>MTQTAAKSLKFPKDFLWGAATAAYQIEGAANEDGRGPSIWDTFSHTPGKVHNGDNGDVACDHYHRYKEDVELMKELGLNAYRFSISWPRILPEGEGKVNQKGLDFYNNLIDELLENGIEPFVTLYHWDLPQALQDKGGWENRETVDAFAEYARVCFERFGDRVKYWITFNEPNVFAVLGYLSGVHPPGMKDLKKAFRAAHNLLLAHARAVKAYREISQNGQIGITLNLSPVYPASDNEEEDKAAAERADQFNNWFLDPIFKGKYEHMLERLGEQIAANGGELPEITDEMEILSASLDFIGLNYYTSNLVRANPNSGSSSVKP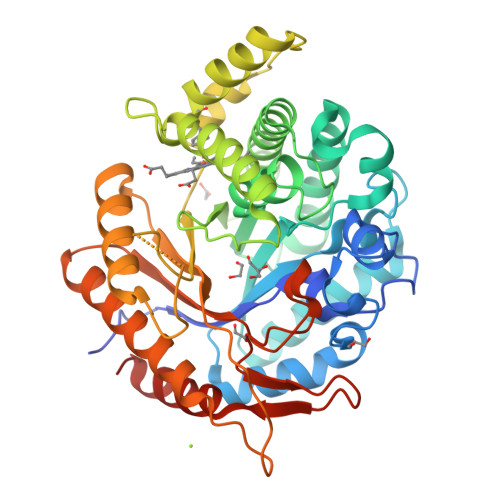PDLPRTDMGWEIYPEGLYDLLKRIHEKYNLPIYITENGMAVDDEVEDGAVHDTNRIDYLKEHLEAVHKAIEEGVNVRGYFVWSLMDNFEWANGYSKRFGLIYVDYKTQKRTPKKSAYWYREVIKSNGLELEHHHHHH[3x]(1R,5S)-6-oxabicyclo[3.1.0]hexane | C5 H8 O | 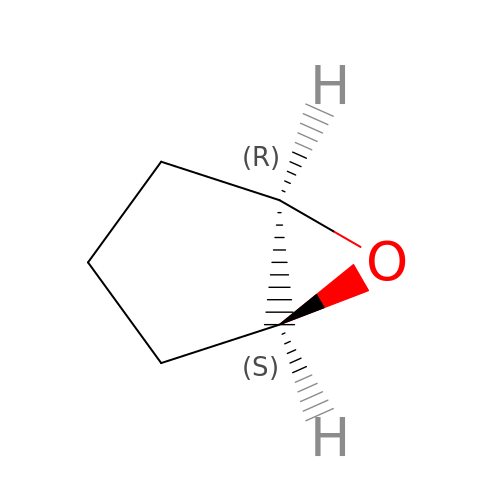GJEZBVHHZQAEDB-SYDPRGILSA-N>[6x]GHMKKPNHSGSGQIRIIGGQWRGRKLPVPDSPGLRPTTDRVRETLFNWLAPVIVDAQCLDCFAGSGALGLEALSRYAAGATLIEMDRAVSQQLIKNLATLKAG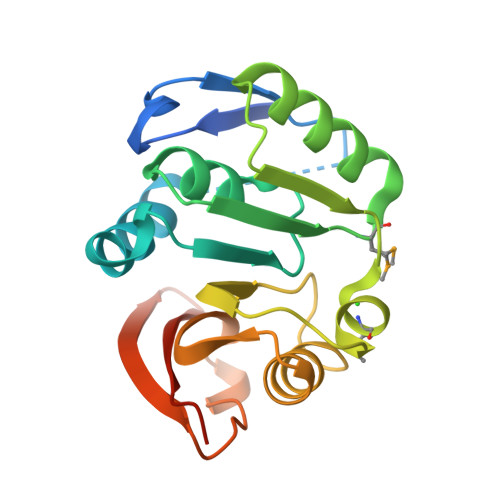NARVVNSNAMSFLAQKGTPHNIVFVDPPFRRGLLEETINLLEDNGWLADEALIYVESEVENGLPTVPANWSLHREKVAGQVAYRLYQREAQGESDADGS> A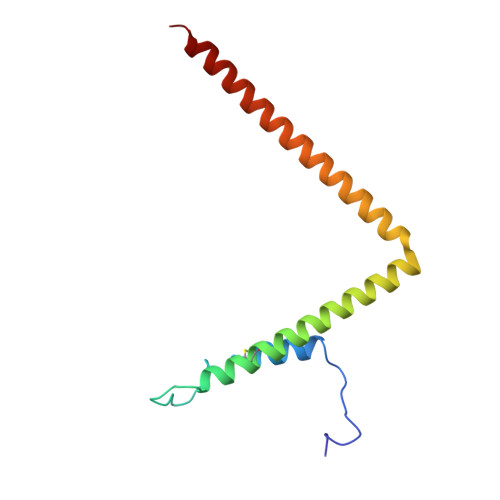APGAPRPSNSTLVDELESSFEACFASLVSQDYVNGTDQEEIRTGVDQCIQKFLDIARQTECFFLQKRLQLSVQKPDQVIKEDVSELRSELQRKDALVQKHLTKLRHWQQVLEDINVQ>MAHHHHHHSSGLEVLFQGPNEQVSRSQQRGLRRVRDLCRVLQLPPTFEDTAVAYYQQAYRHSGIRAARLQKKEVLVGCCVLITCRQHNWPLTMGAICTLLYADLDVFSSTYMQIVKLLGLDVPSLCLAELVKTYCSSFKLFQASPSVPAKYVEDKEKMLSRTMQLVELANETWLVTGRHPLPVITAATFLAWQSLQPADRLSCSLARFCKLANVDLPYPASSRLQELLAVLLRMAEQLAWLRVLRLDKRSVVKHIGDLLQHRQSLVRSAFRDGTAEVETREKEPPGWGQGQGEGEVGNNSLGLPQGKRPASPALLLPPCMLKSPKRICPVPPVSTVTGDENISDSEIEQYLRTPQEVRDFQRAQAARQAATSVPNPP[2x];>[2x]MAHHHHHHSSGLEVLFQGPSGIVPQLQNIVSTVNLGCKLDLKTIALRARNAEYNPKRFAAVIMRIREPRTTALIFSSGKMVCTGAKSEEQSRLAARKYARVVQKLGFPAKFLDFKIQNMVGSCDVKFPIRLEGLVLTHQQFSSYEPELFPGLIYRMIKPRIVLLIFVSGKVVLTGAKVRAEIYEAFENIYPILKG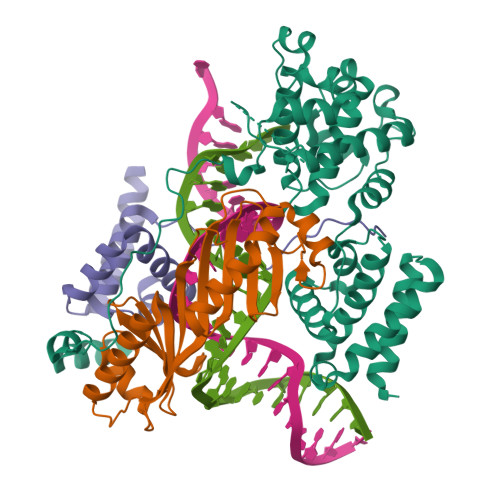FRKTT;>[2x]MAHHHHHHSSGLEVLFQGPGPLLVPRVKVAEDGSIILDEESLTVEVLRTKGPCVVEENDPIFERGSTTTYSSFRKNYYSKPWSNKETDMFFLAISMVGTDFSMIGQLFPHRARIEIKNKFKREEKTNGWRIDKAFQEKRPFDFDFFAHLLQKVLAEEEKRKQKSVKNHSLKEKKS> ENSLSTTSKSKRQVIVPVCMPKIHYSPLKTGLCYDVRMRYHAKIFTSYFEYIDPHPE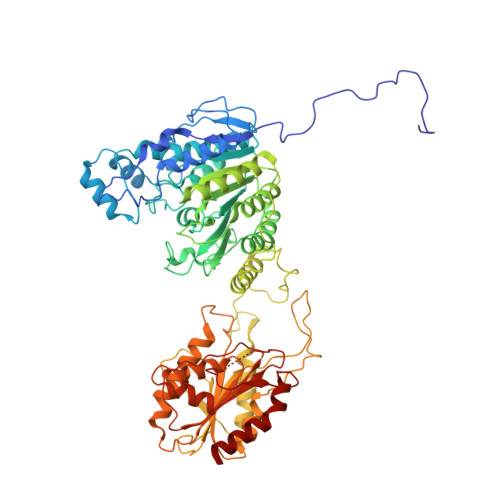DPRRIYRIYKILAENGLINDPTLSGVDDLGDLMLKIPVRAATSEEILEVHTKEHLEFIESTEKMSREELLKETEKGDSVYFNNDSYASARLPCGGAIEACKAVVEGRVKNSLAVVRPPGHHAEPQAAGGFCLFSNVAVAAKNILKNYPESVRRIMILDWDIHHGNGTQKSFYQDDQVLYVSLHRFEMGKYYPGTIQGQYDQTGEGKGEGFNCNITWPVGGVGDAEYMWAFEQVVMPMGREFKPDLVIISSGFDAADGDTIGQCHVTPSCYGHMTHMLKSLARGNLCVVLEGGYNLDAIARSALSVAKVLIGEPPDELPDPLSDPKPEVIEMIDKVIRLQSKYWNCFRRRHANSGCNFNEPINDSIISKNFPLQKAIRQQQQHYLSDEFNFVTLPLVSMDLPDNTVLCTPNISESNTIIIVVHDTSDIWAKRNVISGTIDLSSSVIIDNSLDFIKWGLDRKYGIIDVNIPLTLFEPDNYSGMITSQEVLIYLWDNYIKYFPSVAKIAFIGIGDSYSGIVHLLGHRDTRAVTKTVINFLGDKQLKPLVPLVDETLSEWYFKNSLIFSNNSHQCWKENESRKPRKKFGRVLRCDTDGLNNIIEERFEEATDFILDSFE> HMQHITVRLPKKARAMIVGEITNVFKDKYPIADKLKVIPEYDVIEQDLCKLLSPGFPKQPLRVYKFGSRITGIGNRSSDLDLFVDIGNTFHTFEHRASNATVAKLRAMRKFFCDSEDWRLINFIEQARVPIIKTCHLPTGIECDICLNSMGFCNTNLLKYIFESQPLTQYMCIYVKNWLERCKLTEQISTYSITLMVIYFLQLQALLPPIAMLQIEDAANQAVLVGPWVVNFAQKSFSELGLQQLKATVPVIKGFLRNFFAYFAKFDYEHFLVCPYIGQANVEIAKIERMLHARYSAYVSDNPECSIQLKKPMVVQDPIQLNHNVTKAVTKYGLQTFVDYCQQTAELLEEPSTNWRQRYAF

Terminal uridylyl transferase (TUTase) is one type of enzyme that modifies RNA molecules by facilitating the post-transcriptional addition of uridyl ribonucleotides to their 3′ ends. Recent researches have reported that Drosophila TUTase, Tailor, exhibits an intrinsic preference for RNA substrates ending in 3′G, distinguishing it from any other known TUTases. Through this unique feature, Tailor plays a crucial role as the repressor in the biogenesis pathway of splicing-derived mirtron pre-miRNAs. The structure of Tailor contains two canonical globular domains separated by a large catalytic groove, which serves to accommodate the 3′ ends of the target RNAs for the post-transcriptional addition of uridyl ribonucleotides.

The overall architectures of Tailor in all models are almost identical and resemble the previously reported structures of the other TUTases, belonging to noncanonical nuclear poly(A) polymerase of the DNA polymerase β superfamily. The catalytic domain (CAT) of Tailor consists of a mixed five-stranded β-sheet (β1–β5 strands) packed tightly by two α-helices (h2 and h3) from one side, exhibiting a typical folding of the DNA polymerase β family enzyme. Three conserved catalytic aspartic acid residues (Asp278, Asp280 and Asp 343) sit closely with their side chains all pointing outward from the other side towards the groove. The central domain (CD) of Tailor, on the other hand, is made up of a long α-helix (h1) and a core region of six closely packed α-helices (h4–h9) which is a homologue to the central domain of PAP. The juxtaposed CAT and CD are physically connected through the linkers of h4–β5 and h1–h2. In addition, a highly conserved loop, which has been previously termed as nucleotide-recognition motif (NRM), also exists in the CD of Tailor. Although the overall structures of Tailor in apo and RNA-bound forms are highly similar, careful comparison did reveal a structural perturbation, upon the RNA binding, occurring on a region next to the exit of RNA-binding groove, which is mainly constituted by H294 and R295 from the loop connecting h2 and h3 (L23), R327 from SSL loop, as well as N521 and K525 from NRM loop. Specifically, in RNA-bound structures, the portion of L23 loop (H294 and R295) and SSL loop slightly shifted towards each other upon the RNA binding, forming a direct hydrogen bond between the side-chain of R295 from SSL and the main chain atom of Q325 from L23, which is not observable in the apo-form structure of Tailor. In addition, the side-chain of H294 forms two direct hydrogen bonding interactions with Q519 and N521 while H294 also forms three water-mediated hydrogen bonds with N347, Y500 and N521 using its main chain atoms, in both complex structures. All these H294-related hydrogen bonds were not observed in the apo-form structure of Tailor, reflecting a higher degree of rigidity for this region in the RNA-bound structures, which is consistent with its B-factor profiles in three models.> MTFYEAVGGE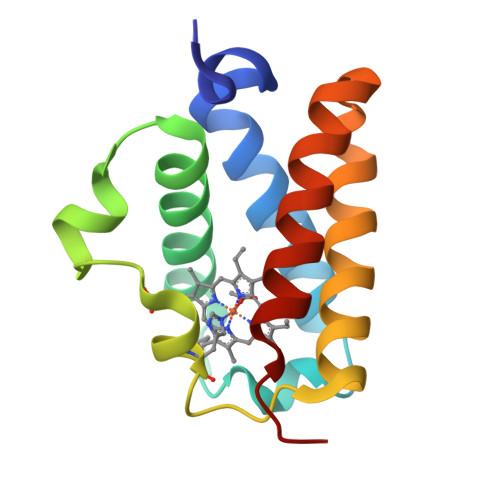ETFTRLARRFYEGVAADPVLRPMYPEEDLGPAEERLRLFLMQYWGGPRTYSERRGHPRLRMRHFPYRIGAEERDRWLTHMRAAVDDLALPAHLEQQLWEYLVYAAYAMVNVPE N-{(2S)-1-({(2S)-1-[(2,4-difluorobenzyl)amino]-1-oxopropan-2-yl}amino)-1,4-dioxo-4-[(2R)-2-phenylpyrrolidin-1-yl]butan-2-yl}-5-methyl-1,2-oxazole-3-carboxamide 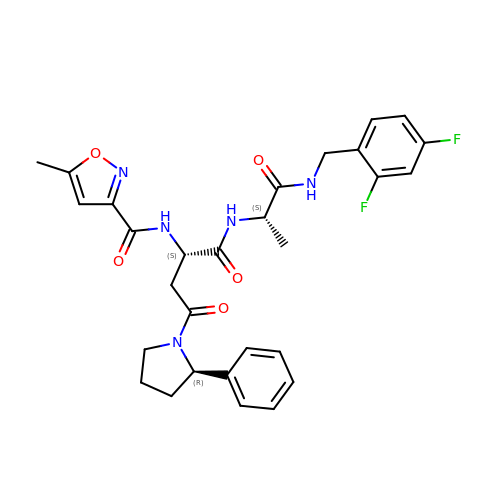(non-preferred name) | C29 H31 F2 N5 O5 | ZUCKFGZJAOBNRP-VVMVZBAXSA-N> MESLPVIAAPSMWTRPQIRDFKEKIRQDSDSVITVGRGEVVTVRVPTHEEGSYLFWEFATDNYDIGFGVYFEWTD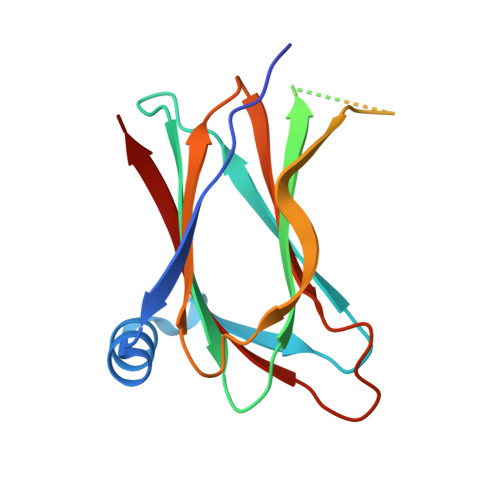SPNTAVSVHVSESSEHDDEEEEENISSEEKAKKNANKPVLDEIVPVYRRDCHEEVYAGSHQYPGRGVYLLKFDNSYSLWRSKSVYYRVYYTR> AGIKVFGHPASIATRRVLIALHEKNLDFELVHVELKDGEHKKEPFLSRNPFGQVPAFEDGDLKLFESRAITQYIAHRYENQGTNLLQTDSKNISQYAIMAIGMQVEDHQFDPVASKLAFEQIFKSIYGLTTDEAVVAEEEAKLAKVLDVYEARLKEFKYLAGETFTLTDLHHIPAIQYLLGTPTKKLFT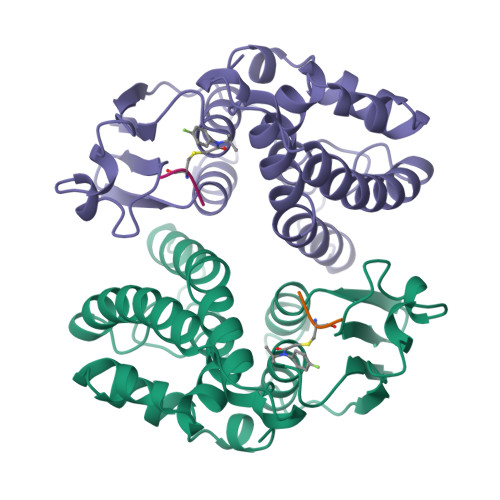ERPRVNEWVAEITKRPASEKVQ;> ECG> 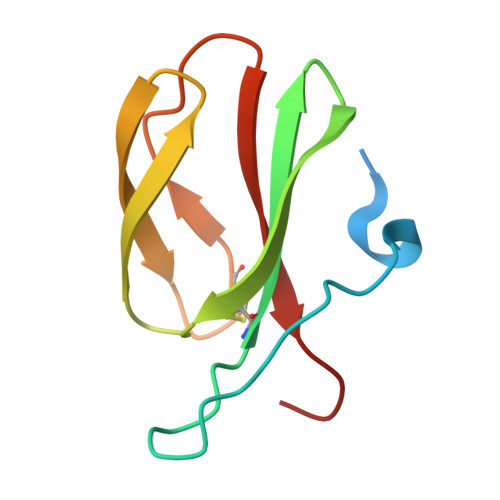METGNKYIEKRAIDLSRERDPNFFDNPGIPVPECFWFMFKNNVRQDDGTCYSSWKMDMKVGPNWVHIKSDDNCNLSGDFPPGWIVLGKKRPGF>GSHMGTSLTDEELVTMSVRELNQHLRGLSKEEIIQLKQRRRTLKNRGYAASCRVKRVTQKEELEKQKAELQ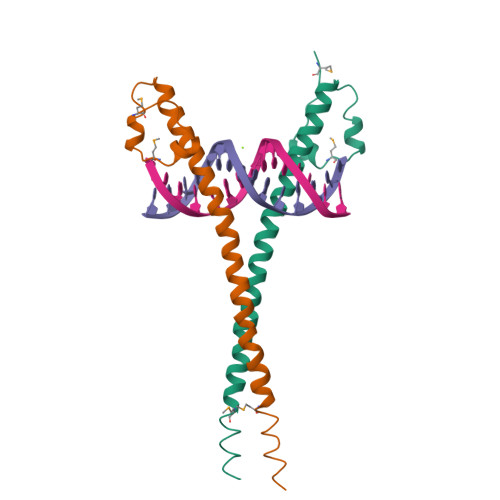QEVEKLASENASMKLELDALRSKYEALQNFARTVAR[2x]> MRRYNTGLFLLSMVMLAGCGKPEVNVVMTGDMTTRLAFAGEQLKQALVEKGYEVNQTTDEKEIGGGKRSIYLNLLNDTTKKNKERFDISTKGKNTYVTGYDGNGIIYGCRELIDQLDQSGTMDFKPVSDAPEMVLRGACIGLQKTTYLPGHAVYEYPYTPESFPWFYDKERWIKYLDMMVENRMNSLYLWNGHPFASLVKLKDYPFALEVDEETFKKNEEMFSFLTTEAEKRGIFVIQMFYNIIVSKPFADHYGIKTQDRNRPITPLISDYTRKSVAAFIEKYPNVGLLVCLGEAIGTYE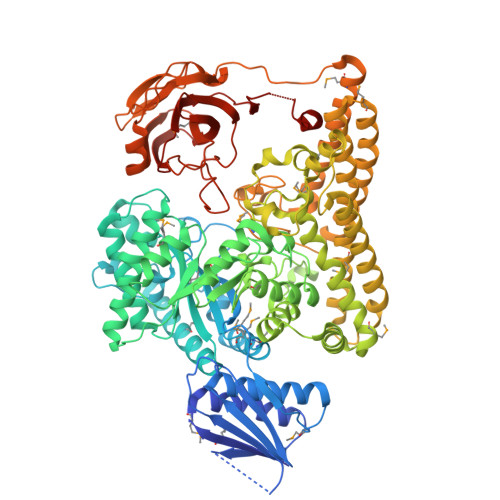EDVEWFTKTIIPGIKDGLKVLGRTDEPPVLVRAHDTDCKMVIDAALPLYKNLYTMHKYNGESLTTYEPRGPWAKIHKDLSSLGSVHISNVHILANLEPWRWSSPDFIQKSVKAMHSVHGANALHIYPQANYWDWPYTADKLANGEREEQVYRDWAWYKAWGRYAWKADRNRLEEIKYWDKQFGDFYGIPAEMADNIRIAYEESGEIAPKLLRRFGITEGNRQTLLLGMFMSQFVNPYKYTIHYGFYESCGPGGEKLIEYVEKEWKKQPHVGELPLDIINQVIEHGDKAVAAIDKVVSSAKKNSDELRRLQNDMHCYREYAYAFYYKVKAAQHVLNYHWGKNMDELDKAVPLMEESLKHYTKLVDLTKDTYLFANSMQTAQRRIPIGGDDGNNKTWSEMLVHYKAELYNFKENIEMLKDKKVRKCVEVTPLKEADVKILNNLTKVKIEKGAKIFSNIDGGIDAIAKEITGLTGFVFNGEKQRDDATTIEFECSSPVTMLVAYFKDDHRKFAKAPRLESDASANDYGQAEPVLTNALHVKGVALADIYPYKFKAGRHTLILPKGYCGVLGFTEDKIKERDVALEGGADAPDWLFY> WMDFDDD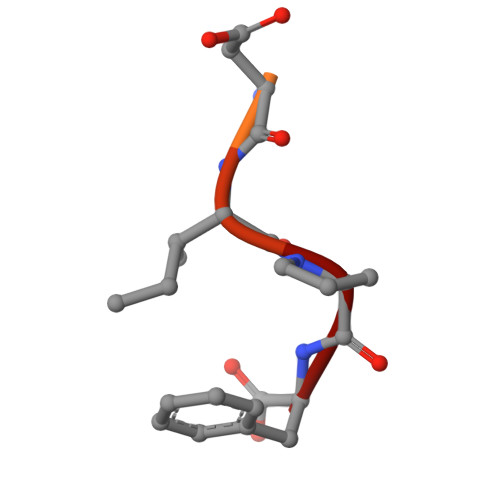IPF>[3x]GVFTFEDEITSTVPPAKLYNAMKDADSITPK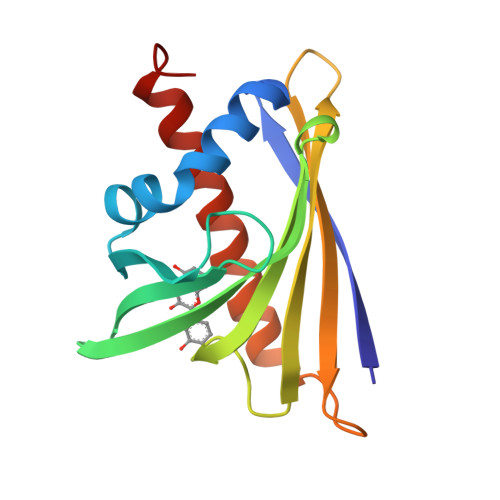IIDDVKSVEIVEGNGGPGTIKKLTIVEDGETKFILHKVESIDEANYAYNYSVVGGVALPPTAEKITFETKLVEGPNGGSIGKLTLKYHTKGDAKPDEEELKKGKAKGEGLFRAIEGYVLANPTQY> GSMGSKRQWALEDFEIGRPLGKGKFGNVYLAREKQSKFILALKVLFKAQLEKAGVEHQLRREVEIQSHLRHPNILRLYGYFHDATRVYLILEYAPLGTVYRELQKLSKFDEQRTATYITELANALSYCHSKRVIHRDIKPENLLLGSAGELKIADFGWSVHAPSSRRTTLCGTLDYLPPEMIEGRMHDEKVDLWSLGVLCYEFLVGKPPFEANTYQETYKRISRVEFTFP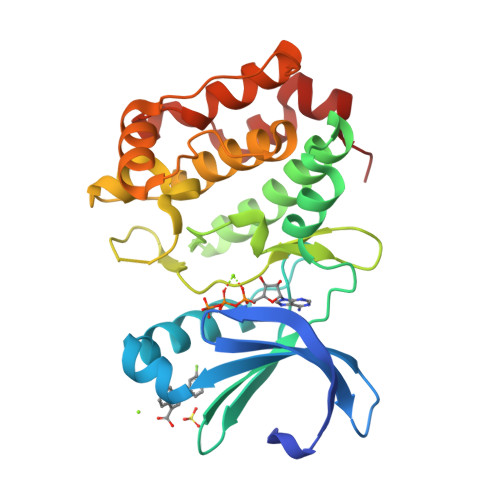DFVTEGARDLISRLLKHNPSQRPMLREVLEHPWITANSSKPS>FVNRGGLPVDEATWERMWKHVAKIHPDGEKVAQRIRGATDLPKIPIPSVPTFQPSTPVPERLEAVQRYIRELQYNHTGTQFFEIKKSRPLTGLMDLAKEMTKEALPIKCLEAVILGIYLTNSMPTLERFPISFKTYFSGNYFRHIVLGVNFAGRYGALGMSRREDLMYKPPAFRTLSELVLDFEAAYGRCWHVLKKVKLGQSVSHDPHSVEQIEWKHSVLDVERLGRDDFRKELERHARDMR[2x];>KSAQQELKQRQRAEIYALNRV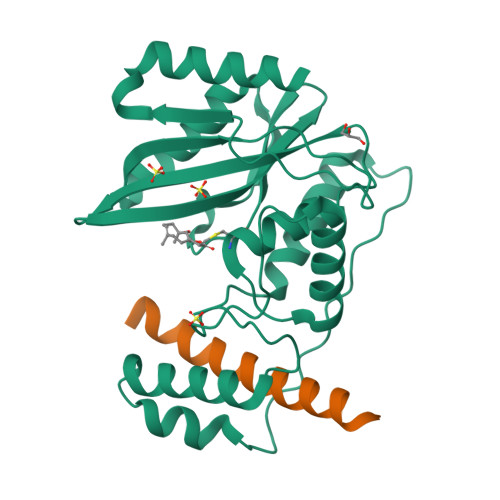MTELEQQ[2x]> MKRRSLKGIALFLLIVAVCLSSATLGRGEEKHTGENVRQNQKVKDPQFTNVSVHDPSIVKDGDTYYIFGSHIEAAKSKDLMNWEKFTNGYTTPNNKLYGDLSKNLAGSFKWAGENDADSKGGFAVWAPDVFWNKDYVNEDGTKGAYMIYYSVSSTYIRSAIGYAVSKHIEGPYKYVDTIVYSGFTKEEAYDANSKINKKWTNTNIPKLIEQGKLKGVRADWFHNDGSYNNRDFPNAIDPNLFYDEKGNLWMAYGSWSGGIFVLPMDKTTGKPIYPGKDGKTPDGRLVDRYFGIKIAGGYYQSGEGTYIVYDKNTDYYYLYVTYGWLGADGGYNMRQFRSTSPTGPYVDAKGQSAVLPGEVDNSPYGNKIMGNFLFERKVGDPGTGIGVGYVSPGHNSVYLDRKTGQQFLVFHTRFPQSGEYHEVRVHQMFMNKNGWPVVAPYRYAGEKLEKVNKQDVVGEYQLINHGKDYSADIKKQIFVRLNRNNTISGDATGTWRKIGHNQAEITIDGETYDGVFVRQWDPTSKRYVMAFTALSNEGVSIWGSKLADKTDEEIVEDVASDLDLGDTDHVVSNL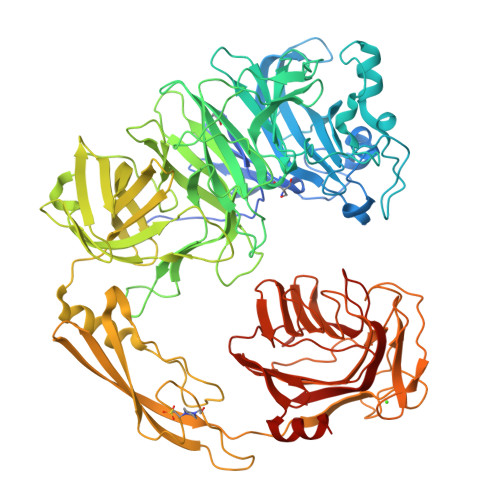HLPTEGTRHTVISWTTSDAKVVSETGVVHRPEVGSAPVTATLTATITKGDATATKVFHITVLPYEEAKLTAHYSFDNNDLSDSTGNFGPGTITGNRIDNEGGTIAYADGKIGKAAVLNGQSGIRLPDGLVSSNQYSVSLWVKPEQLTTHTTTFFGAKDPNHWISLVPQGWDGNTMLWSGSSPWYDGRTFWKIPTGQWTHLAFSVDNGAVKVYINGVEKFSGTNFPDVFTGANASFALGVNWWDPPFKGLIDELRIYEGALTPSQVTDLAQTSE(7R)-2-[(3,5-difluoro-4-hydroxyphenyl)amino]-7-methyl-8-(3-methylbutyl)-5-(prop-2-yn-1-yl)-7,8-dihydropteridin-6(5H)-one | C21 H23 F2 N5 O2 | 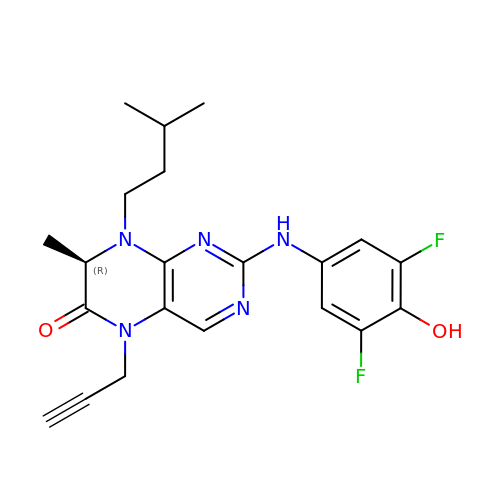IHZPRIAIJQSUAF-CYBMUJFWSA-N>MRGSHHHHHHGSMPVAGSELPRRPLPPAAQERDAEPRPPHGELQYLGQIQHILRCGVRKDDRTGTGTLSVFGMQARYSLRDEFPLLTTKRVFWKGVLEELLWFIKGSTNAKELSSKGVKIWDANGSRDFLDSLGFSTREEGDLGPVYGFQWRHFGAEYRDMESDYSGQGVDQLQRVIDTIKTNPDDRRIIMCAWNPRDLPLMALPPSHALCQFCVVNSELSCQLYQRSGDMGLGVPFNIASYALLTYMIAHITGLKPGDFIHTLGDAHIYLNHIEPLKIQLQREPRPFPKLRILRKVEKIDDFKAEDFQIEGYNPHPTIKMEMAV[4x]

Human thymidylate synthase (hTS) is an obligate, stable homodimer (Kd = 80 nM Genovese et al., 2010) with two active sites, each including residues from both monomers. As a dimeric enzyme, it provides the sole de novo pathway to deoxythymidylate (dTMP) synthesis in human cells by catalyzing the reductive methylation of deoxyuridylate (dUMP) to dTMP using methylenetetrahydrofolate (mTHF) as the one-carbon methyl donor. By interacting with its own and other mRNAs, this protein regulates its own levels and those of other proteins involved in apoptotic processes, including bcl2, c-myc, and p53. Its inhibition is usually achieved with compounds that bind at the protein active-site, competing either with the dUMP substrate, such as 5-fluorodeoxyurdine 5’-monophosphate (FdUMP), or with the folate cofactor, such as raltitrexed (RTX) and pemetrexed (PMX) (Carreras and Santi, 1995; Jennings and Willis, 2015). Here we report the discovery of molecules that bind at the hTS monomer/monomer interface and, despite their small size, markedly shift the monomer-dimer equilibrium of the enzyme towards the inactive monomeric form.

To target the monomer-monomer interface and dissociate the hTS dimer, we applied the ‘cysteine tethering’ approach to fragment-based drug design. We selected the ‘Y202 pocket’, which accommodates the side chain of F59’ from the other monomer, as the most promising region to target (Salo-Ahen et al., 2015). We therefore made the Y202C mutant and screened for compounds able to form a covalent disulfide bond with C202 from a library of organic disulfides. We also mutated the active site cysteine to serine to prevent the selection of compounds that bound at the active site (C195S). We made mutants with single point mutations at C195S and Y202C to test their functional and structural properties as well as the double mutant, hTS C195S-Y202C. This was used for the ligand selection according to the above-described tethering approach. As expected from removal of the catalytic C195 residue, this double mutant was inactive, but X-ray crystallography showed that it takes the active conformation of hTS. We employed the C195S-Y202C double mutant to capture compounds that, driven by some affinity for the region near residue 202, formed a covalent disulfide bond with C202. (a–c) Unbiased omit map (blue wired map contoured at 3.0 σ), showing the S,S(2-hydroxyethyl)cysteine (CME) chemical modification occurring at the mutated residue C202, and the mutated residue S195 in the hTS double mutant C195S-Y202C. Four molecules, A5, A10, A20, and TPC also bound peptide (D186-R215) DLPLMALPPSHALCQFCVVNSELSCQLYQR (sequence C), containing the engineered Y202C together with the native C199 and C210. In agreement with the described computational and crystallographic data (see above), Y202C is the most exposed of these three cysteines and is thus easily available for disulfide-bond formation with the RS fragments, being therefore suitable for tethering experiments.>HHHHHHPCCSNPCQNRGECMSTGFDQYKCDCTRTGFYGENCTTPEFLTRIKLLLKPTPNTVHYILTHFKGVWN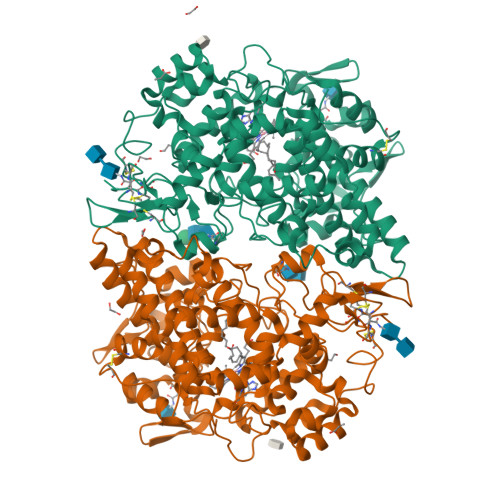IVNNIPFLRSLIMKYVLTSRSYLIDSPPTYNVHYGYKSWEAFSNLSYYTRALPPVADDCPTPMGVKGNKELPDSKEVLEKVLLRREFIPDPQGSNMMFAFFAQHFTHQFFKTDHKRGPGFTRGLGHGVDLNHIYGETLDRQHKLRLFKDGKLKYQVIGGEVYPPTVKDTQVEMIYPPHIPENLQFAVGQEVFGLVPGLMMYATIWLREHNRVCDILKQEHPEWGDEQLFQTSRLILIGETIKIVIEDYVQHLSGYHFKLKFDPELLFNQQFQYQNRIASEFNTLYHWHPLLPDTFNIEDQEYSFKQFLYNNSILLEHGLTQFVESFTRQIAGRVAGGRNVPIAVQAVAKASIDQSREMKYQSLNEYRKRFSLKPYTSFEELTGEKEMAAELKALYSDIDVMELYPALLVEKPRPDAIFGETMVELGAPFSLKGLMGNPICSPQYWKPSTFGGEVGFKIINTASIQSLICNNVKGCPFTSFNVQDPQPTKTATIAASASHSRLDDINPTVLIKRRSTEL[2x]methyl 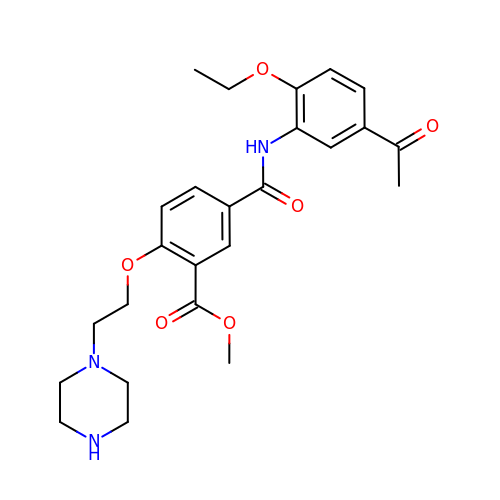5-[(5-ethanoyl-2-ethoxy-phenyl)carbamoyl]-2-(2-piperazin-1-ylethoxy)benzoate | C25 H31 N3 O6 | LQHWWGHAUAZICR-UHFFFAOYSA-N>MKSSHHHHHHENLYFQSNAEESAQQRSERYVSARSQHPAWLLLASRRAPLVLGCLRTLFERAHDGIPMEDALQALSEMLAAYASQELYEIDPDATHLQAGRELREWIKRRLVVEREGRIYATDALESAIQFVDSLDSRIMTSTASRLSVVQREIENLETGLNPSPTGRIASLRRRIQDLEHELARVEAGHVDVLDEAQAIEGMREVYNLATSLRADFRRVEDSWREADRALRHSIISEQSHRGEIVDRLLDGQDALLNTPEGRVFESFQQQLRQSAELEVMRERLRTILRHPAVPKALNRPQQRELRWLALRLVRESQAVLQARARSERDVRGFMKTGLAAEHHRVGQLLNDFFNLALSVDWQRQSERRKPACLPPVGVAITGVPAIERLRFKTLDDDDAGELDLSLKPAGLEQIDDDFWDAFDGLDREALIHDTLAVLVEQGRPVSLGELASLLPPAHDLETFALWLAMAREAGIEVLTEERQFVELVDEDEQRWGFNLPYVGLDHEALKDIDWEL[2x];>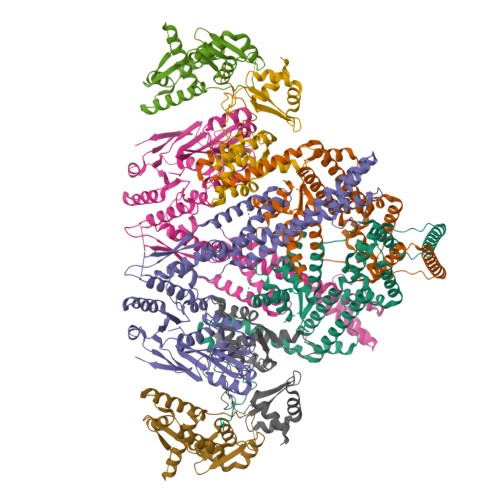MKSSHHHHHHENLYFQSNAKQALLWRDSETFILTSIELYNWGGFQGYHRAEIDPSGTAVIGPTGSGKTTLVDALMTLLCANPRYNLASTGGHESDRDLVSYVRGVTGPGDGGVEQSHIARQGKTVTAIAATLERDGAQVRLGAVLWFEGTSSSASDLKKLWLLSESPEQTLEHWLSQHHAGGMRALRQMEKDGMGIWPYPSKKAFLARLRDYFEVGENAFTLLNRAAGLKQLNSIDEIFRELVLDDRSAFERAAEVASSFDDLTDIHRELETARKQQRSLQPVADGWERYRALQEQLQDKQASGSSGSSGSSGQAKTLGEKLGDQKTELAKRMSDALKADTGALAEVGRELVDVPRYLERLRVLTEEALPEKLKRFLEYLNRSSDDGVTQLLSYIDHEVSMIEERLDDLNSTMQRVDFQPGRYLRLVAKKVIHESLRTLQHAQRQLNSARFIDDEGESHYKALQALVGLLKDACEHSRNQGAKALLDPRFRLEFAVSVIDREGNNLIETRTGSQGGSGGEKEIIASYVLTASLSYALCPDGSSRPLFGTIVLDQAFSRSSHAVAGRIIAALREFGLHAVFITPNKEMRLLRHHTRSAVVVHRRGVESSLVSLSWEALDEHHQQRIRAMHEVAH[2x];>[4x]MAGIFDRIAGASGADETELTAEPMALDDGMDGEQPAMSANIQVDERRTPQRVREAVQEMLKYGLLEESHKPNLYRSALTNIEVVDRILEPLDLAMGVDEVRGLVFVTVRQGEVAEQDDWSHPLVRRQRLNLEQSLLIAILRQHFIAYEQESGTGASQALVAVDELIPQLQVYLGELGSEAKERNRIITLLDQLKGHGLVSALDAHDRVIIRPIITHLANPENLQALVVWLREQVEGAVTPAAGGEEDEA>[2x]GSHMAKTVILDHDGNKDDFVAMILLLSNPKKVNLIGCICTDADCFVENGFDVTGKIMCAMHRLIKTPLFPIGKSTATAVNAFPTEWRFSAKNLDDMPFLNIVEDVALWEKLKPENEAHNGQQLLADLVMKSKEKVTVCVTGPLSNMAWCIEKYGEAFTSKVEECVIMGGAVDVGGNVFLPTTDGSAEWNIYWDPPAAKKVL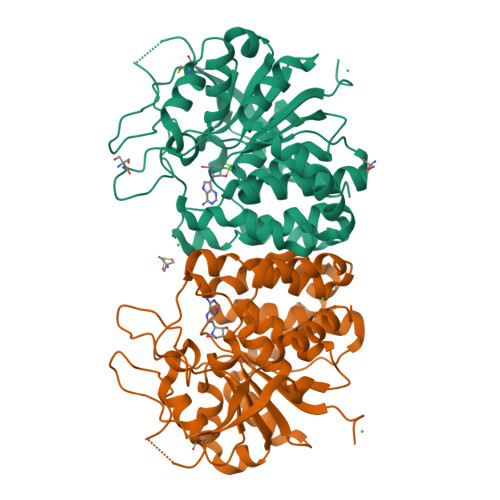CCPNIRCVLFSLDATNTVPVRSVDVKGFGAQNQYLLSQMVGTMWAMSTHEEILRDGDAYYAWDALTAAYILEPTIATLEPVALDVDVSKGKSEGRTPRASGEGKPCVHVARNPSKQMFHDLVFASTRVC>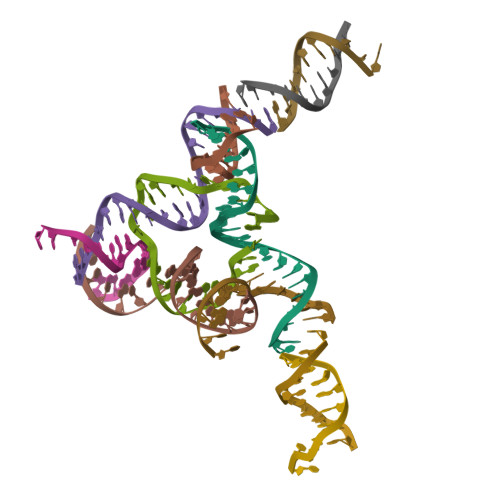 CACGAGCCTGATCGGACAAGA;> AGGCAGCCTGTACGGACATCA;> AACCTACCTGGCAGGACGACT;> GATCTTGTGGCTGC;> TTAGTCGTGGCTCG;> ACTGATGTGGTAGG;> TCACCTGCCACCGTACACCGA;> TCCGCTAGCG;> TGCGCTAGCG;> GTCTATGCTA;> CTTAGCATAG[4-[(3-chloranyl-4-imidazolidin-2-ylideneazaniumyl-phenyl)carbamoyl]phenyl]-imidazolidin-2-ylidene-azanium 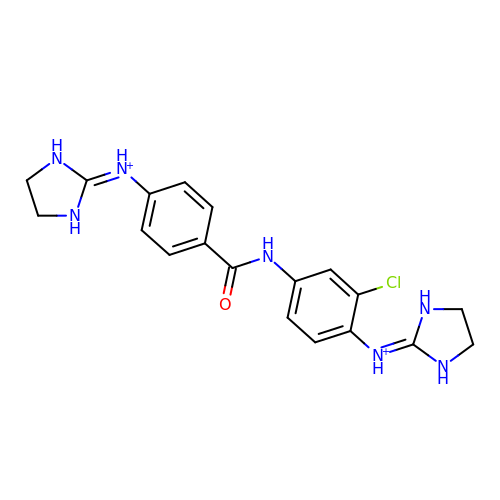| C19 H22 Cl N7 O | RZRDBTPEIPCUHV-UHFFFAOYSA-P> MPSYLSPGVYVEEVASGSRPIEGVGIEGVGTSVAAFVGLAPTGPLNEPTLVTNWTQYVAAFGDFTGGYYLAHSVYGFFNNGGSAAYVVRVGGSAEDAAADGSVNGAAAPAAVTGSTAKALPAAEPKQLGTFAVTATAAGQSGPLTVEVADPEGEGPAERFKLIVKDGDKPVETFDVSAKKGNRSYVVTQVKERSKLITVTEAAPSAQLVRPENQSLTLPAPPSAAPAVPAGQAESAHPGPAQYLGDSSDRTGFGGLEAIDEISMVAVPDLMAAYQRGAIDLEAVKAVQLGLIAHCELMGDRVAIIDPPPNQNARQIRVWRQETAGYDSKYAALYYPWIKSFDPATGQSRLVPPSGHVAGIWARNDSERGVHKAPANEVVRGAVDLELQITRGEQDLLNPIGVNCIRSFPGRGIRVWGARTLSSDPAWRYLNIRRYFNYLEESILIGTQWVVFEPNDHNLWARIRRNV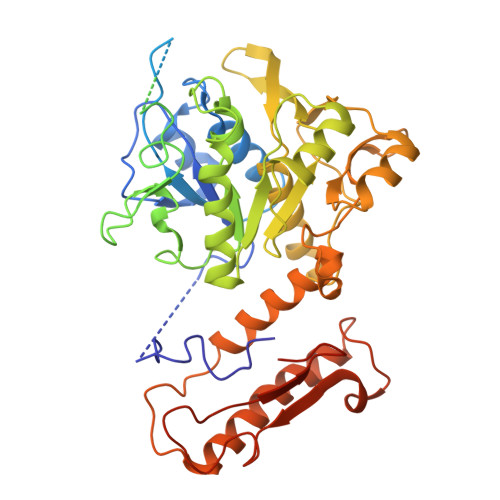SAFLVNEWRNGALFGQSPDQAYYVKCDEETNPPESVDLGRVVCEIGIAPVKPAEFVIFRLAQFSSGGGELDE The ferrous iron and 2-oxoglutarate (2OG)-dependent HIF prolyl hydroxylases (PHDs/EGLNs) catalyse trans-4-prolyl hydroxylations on HIFα subunits, thus promoting their binding to the von Hippel–Lindau protein (VHL), a targeting component of a ubiquitin E3 ligase, and signalling for HIFα degradation under normoxic conditions. The PHD-catalysed hydroxylations of HIF-1α/HIF-2α in higher animals occur in amino- and carboxy-terminal oxygen-dependent degradation domains (NODD and CODD). The three human PHDs exhibit different NODD/CODD selectivities, with PHD3 being substantially more selective for CODD than PHD1/2 (refs 16). Biophysical analyses employing crystallography and NMR reveal that the molecular basis of PHD isoform and variant selectivity involves enzyme–substrate interactions involving β2/β3 loop residues (that bind the LXXLAP motif) and helices α3 and α4, regions which display sequence variations between the PHD isoforms.

We obtained a PHD2.2OG.CODD structure using the strategy used for the PHD2.NOG.CODD complex, but did not obtain PHD2.NODD crystals using this procedure, possibly because NODD binds PHD2 less tightly, as indicated by a lower dissociation rate constant (kd) for CODD compared with NODD29. We then used a ‘disulfide cross-linking' strategy to form stable PHD2.Mn.NOG.NODD complexes, where PHD2QM1 (C201A/P317C/R281C/R398A) or PHD2QM2 (C201A/V314C/R281C/R398A) and NODDDC (L397C/D412C) are cross-linked via appropriately positioned cysteines. Molecular dynamics (MD) simulations predict the PHD2.Fe. OG.NODD solution structure is very similar to that of the disulfide-linked complex, PHD2QM1.Mn.NOG.NODDDC (or PHD2.NODD). Comparison of the ODD complex structures and those without substrate reveals clear differences in NODD/CODD binding, especially in β2/β3 loop and C-terminal regions. NODD makes more hydrophobic contacts than CODD with the C-terminal region of PHD2. However, an important difference between NODD and CODD binding is that in contrast to CODD, substantially less perturbation was observed in the helix α4 with NODD, supporting the crystallography, that is, α4 adopts similar conformations whether bound to NODD or not.

>GSHMASPNGQTKPLPALKLALEYIVPAMNKHGICVVDDFLGKETGQQIGDEVRALHDTGKFTDGQLVSQKSDSSKDIRGDKITWIEGKEPGCETIGLLMSSMDDLICHCNGKLGSYKINGRTKAMVACYPGNGTGYVRHVDNCNGDGRCVTCIYYLNKDWDAKVSGGILRIFPEGKAQFADIEPKFDRLLFFWSDRRNPHEVQPAYATRYAITVWYFDADERAAAKVKYLTGEKGVRVELNKPSDSVGKDVF[2x];>[2x]DACTLLAPAAGDTIISLCF>GSMAAQRRSLLQSEQQPSWTDDLPLCHLSGVGSASNRSYSADGKGTESHPPEDSWLKFRSENNCFLYGVFNGYDGNRVTNFVAQRLSAELLLGQLNAEHAEADVRRVLLQAFDVVERSFLESIDDALAEKASLQLERLKTLEREISGGAMAVVAVLLNNKLYVANVGTNRALLCKSTVDGLQVTQLNVDHTTENEDELFRLSQLGLDAGKIKQVGIICGQESTRRIGDYKVKYGYTDIDLLSAAKSKPIIAEPEIHGAQPLDGVTGFLVLMSEGLYKALEAAHGPGQANQEIAAMIDTEFAKQTSLDAVAQAVVDRVKRIHSDTFASGGERARFCPRHEDMTLLVRNFGYPLG[2x];>[2x]GSHMKTCVPADINKEEEFVEEFN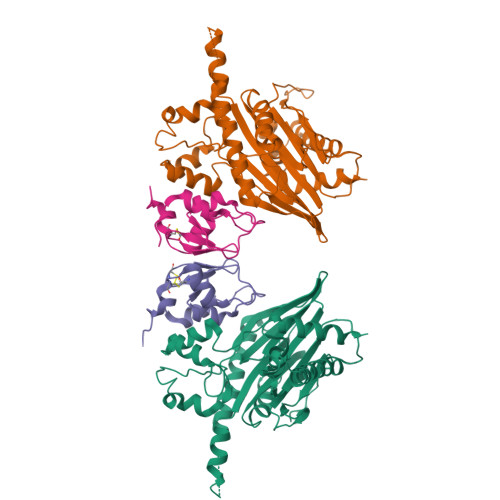RLKTFANFPSGSPVSASTLARAGFLYTGEGDTVRCFSCHAAVDRWQYGDSAVGRHRKVSPNCRFINGFYLEN> PQLPEVETIRRTLLPLIVGKTIEDVRIFWPNIIRHPRDSEAFAARMIGQTVRGLERRGKFLKFLLDRDALISHLRMEGRYAVASALEPLEPHTHVVFCFTDGSELRYRDVRKAGTMHVYAKEEADRRPPLAELGPEPLSPAFSPAVLAERAVKTKRSVKALLLDCTVVAGFGNI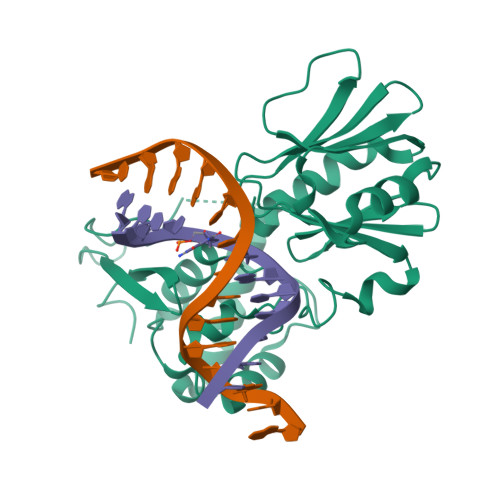YVDESLFRAGILPGRPAASLSSKEIERLHEEMVATIGEAVMKGGSTVRTYVNTQGEAGTFQHHLYVYGRQGNPCKRCGTPIEKTVVAGRGTHYCPRCQR>[5x]MEFLMSKHEADAPHLLIVEARFYDDLADALLDGAKAALDEAGATYD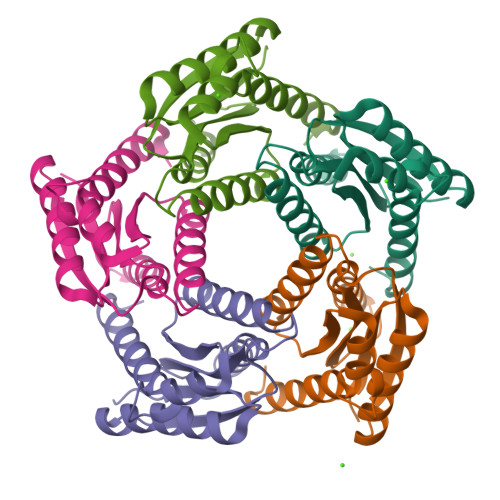VVTVPGALEIPATISFALDGADNGGTEYDGFVALGTVIRGETYHFDIVSNESCRALTDLSVEESIAIGNGILTVENEEQAWVHARREDKDKGGFAARAALTMIGLRKKFGA>PCCELITNISIPDDKAQNALSEIEDAISNVLGKPVAYIMSNYDYQKNLRFSGSNEGYCFVRLTSIGGINRSNNSSLADKITKILSNHLGVK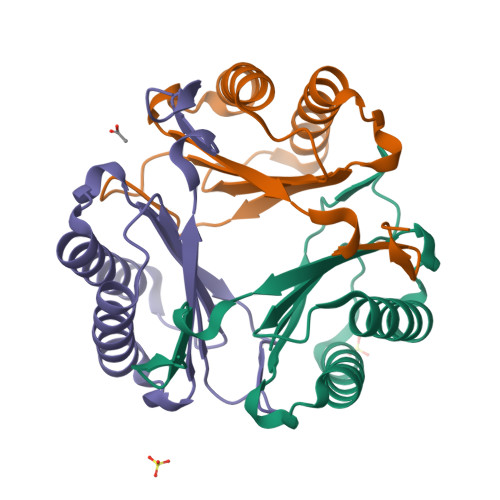PRRVYIEFRDCSAQNFAFSGSLFGLE[6x]>SAKDERAREILRGFKLNWMNLRDAETGKILWQGTEDLSVPGVEHEARVPKKILKCKAVSRELNFSSTEQMEKFRLEQKVYFKGQCLEEWFFEFGFVIPNSTNTWQSLIEAAPESQMMPASVLTGNVIIE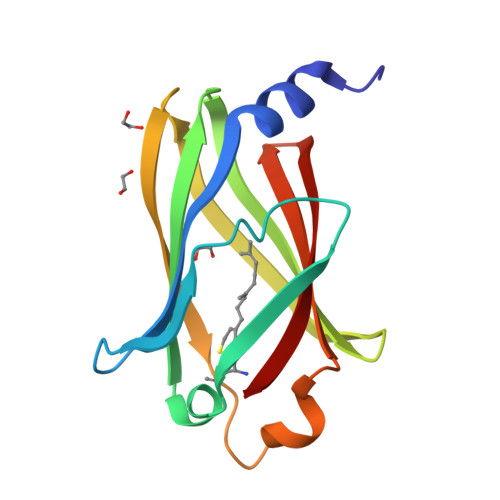TKFFDDDLLVSTSRVRLFYV[2x];> SGPGCMSCKC>MASYPKLTGTVIGTQGSWNNIGNTIHKAFDGDLNTFFDGPTANGCWLGLDFGEGVRNVITQIKFCPRSGYEQRMI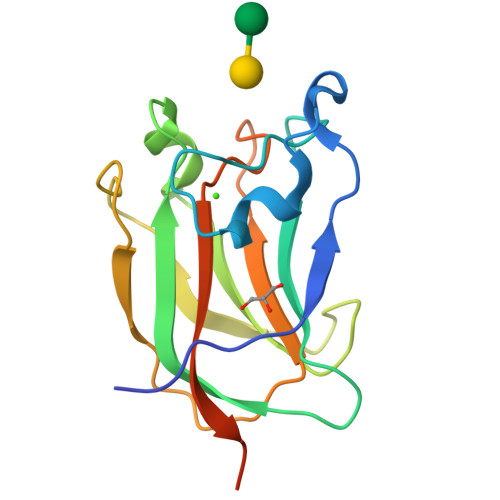GGIFQGANKEDFSDAVTLFTITSLPGSGTLTSVDVDNPTGFRYVRYLSPDGSNGNIAELQFFGTPAGEENDDLEHHHHHH[2x]> VCNRLEQILVKTQWAQSYGEAENRAAFSRDLFSELFNIQGSSRALFSGVGVDDMNSAAFTAHCLRVTGALNRLISQLDQQATIN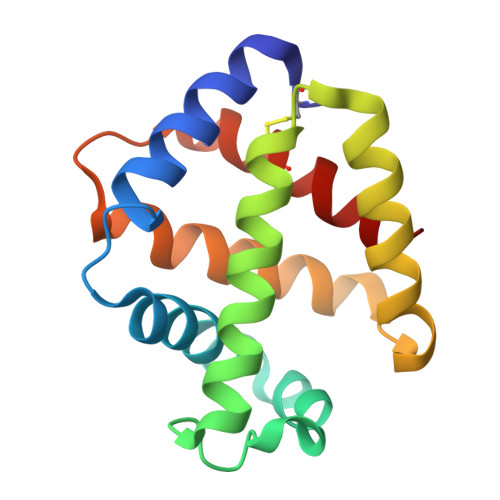ADLAHLAGQHASRNLDASNFAAMGQAVMSVVPTHLDCFNQHAWGECYERIASGISG>[4x]MATQGVFTLPANTRFGVTAFANSAGTQTVNVLVNNETAATFSGQSTNNAVIGTQVLNSGSSGKVQVQVSVNGRPSDLVSAQVILTNELNFALVGSEDGTDNDYNDAVVVINWPLG

The present study is devoted to the PA-IIL lectin from Pseudomonas aeruginosa, an opportunistic human pathogen capable of causing lethal complications in cystic fibrosis patients. The lectin may play an important role in the process of virulence, recognizing specific saccharide structures and subsequently allowing the bacteria to adhere to the host cells. It displays high values of affinity towards monosaccharides, especially fucose – a feature caused by unusual binding mode, where two calcium ions participate in the interaction with saccharide. Briefly, the structure is tetrameric with each monomer characterized by a binding site containing two calcium ions and a saccharide.

All crystal structures belong to the P21 space group except for the S23A mutant that crystallizes in space group C2. Hence, amongst the four monomers that form the asymmetric unit, substitution of the sugar occurred in the four monomers of PA-IIL S23A/Me-α-Fuc and G24N/Me-α-Man, but only in three monomers of the S22A/Me-α-Man and S22A/Me-α-Fuc complexes and in only two monomers of G24N/Me-α-Fuc. In case of mutation of Ser23 to Ala23, the original hydrogen bond between Ser22 and Asp96 is retained. A new hydrophobic interaction is enabled between the methyl group at O1 of the fucoside and the side chain of Ala23. Mutant S23A is even more interesting. The affinity towards methyl fucoside is almost two times higher than in the case of the native protein. The native protein displays an unfavourable entropic contribution TΔS of -4.9 kJ/mol, whereas the mutant shows a favourable entropic part of 3.8kJ/mol, making the total difference 8.7kJ/mol. The hydroxyl group of Ser23 in the native protein interacts with the fucoside O5, creating an unfavourable entropy contribution. If this interaction was absent, the entropic contribution would become favourable for the free energy and consequentially, for the affinity. By replacing Ser23 with alanine, another interaction is also generated: the hydrophobic interaction between the side chain of alanine and the C5 methyl group of fucose.>MENTENSVDSKSIKNLEPKIIHGSESMDSGISLDNSYKMDYPEMGLCIIINNKNFHKSTGMTSRSGTDVDAANLRETFRNLKYEVRNKNDLTREEIVELMRDVSKEDHSKRSSFVCVLLSHGEEGIIFGTNGPVDLKKITNFFRGDRCRSLAGKPKLFIIQACRGTELDCGIETD[2x];>SGVDDDMACHKIPVEADFLYAYSTAPGYYSWRNSKDGSWFIQSLCAMLKQYADKLEFMHILTRVNRKVATEFESFSFDATFHAKKQIPCIVSMLTKELYFYHL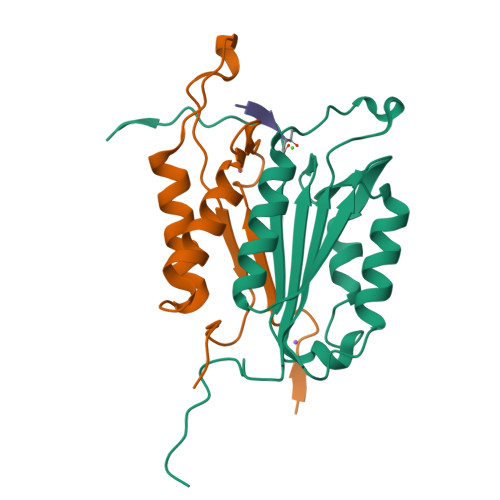[2x]>LYIQWL[2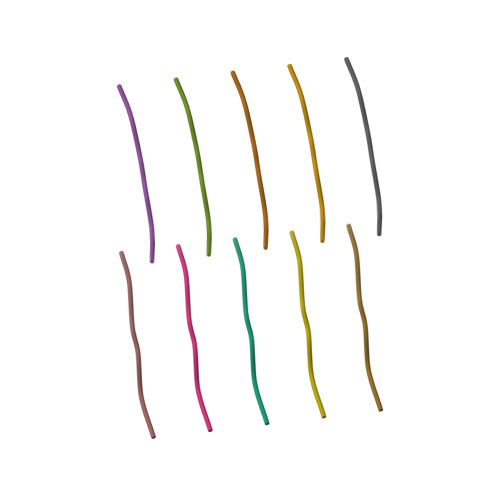x]>[2x]MVGLADVAVLYSGGKDSNYALYWAIKNRFSVKFLVTMVSENEESYMYHTINANLTDLQARALGIPLVKGFTQGEKEKEVEDLKRVLSGLKIQG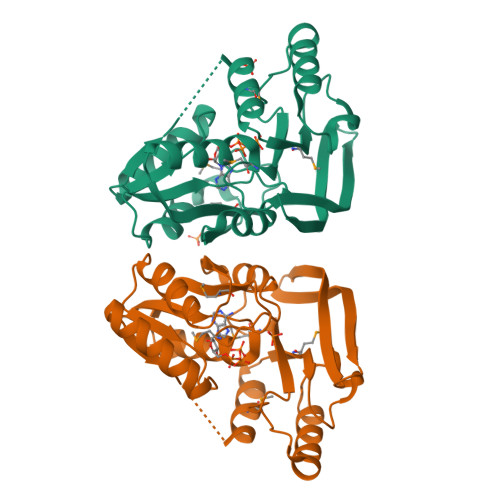IVAGALASKYQRKRIEKVAKELGLEVYTPAWGRDAKEYMRELLNLGFKIMVVGVSAYGLDESWLGRILDESALEELITLNEKYKVHVAGEGGEFETFVLDMPLFKYKIVVDKAKKVWEPCTSSGKLIIEEAHLESKLEHHHHHH>KKPKLLYCSNGGHFLRILPDGTVDGTRDRSDQHIQLQLSAESVGEVYIKSTETGQYLAMDTDGLLYGSQTPN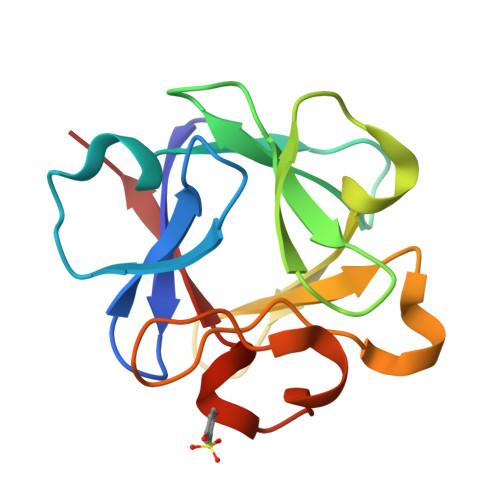EECLFLERLEENHYNTYISKKHAEKNWFVGLKKNGSCKRGPRTHYGQKAILFLPLPVS[6x]2-[(phenylmethyl)carbamoylamino]benzoic acid | C15 H14 N2 O3 | 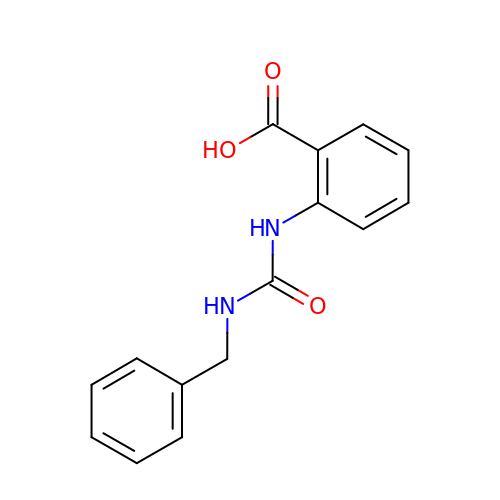QCLRLHJAKXQKSY-UHFFFAOYSA-N>[2x]MAHHHHHHVDDDDKMVHHDGFQTVKATIDWEHPMFKLYEKAKRNGKWNPADIDFSQDQKDFASLTSEEKISALPLVAGFSAGEEAATLDILPMAHALARQGRLEDVLFLTTFMHDEAKHVEMFSRWQQAVGIGQMDLSVFHNDHYKRIFYEALPEAMNRLYADDSPEAVIRAATVYNMIVEGTLAESGYYTFRQIYKKAGLFPGLLQGIDYLNMDEGRHIQFGIYTIQRIVNEDERYYELFIRYMDELWPHVIGYVDYLTELGKRQQQLARTYALEIDYDLLRHYVIKQFNLRKKQISRTKRVDVVEGLEKTAAES

The heterodinuclear Mn/Fe cofactor is found in the R2 subunits of subclass Ic ribonucleotide reductases (denoted as R2c) as well as a related group of proteins known as R2-like ligand-binding oxidases (R2lox). Although the physiological function of R2lox proteins is not known, the cofactor catalyzes formation of a tyrosine–valine ether cross-link in the protein scaffold. Two proteins from this group have been characterized to date, homologs from Mycobacterium tuberculosis and Geobacillus kaustophilus. Both contain the ether cross-link, and both co-purify from heterologous expression hosts with a long-chain fatty acid ligand bound in a hydrophobic channel leading from the protein surface to the active site, hence the name ligand-binding oxidase. The two metal ions are bound next to each other in octahedral geometry by two histidines and four glutamates, with the manganese ion occupying the N-terminal metal-binding site 1.

The cross-linking valine, which is completely conserved across the R2lox group, was changed to an alanine, isoleucine or leucine (V72A/I/L). Crystal structures were obtained of all three R2lox point mutants in the non-activated reduced and the oxidized resting state by soaking apo-protein crystals with MnII and FeII under anoxic or aerobic conditions, respectively. The V72A/L mutations were found to have little effect on the global structures of the reduced and oxidized resting states, but an ether cross-link was not formed in the oxidized state. The mutations affect the position of the fatty acid ligand in comparison to the wild-type, likely due to decreased or increased steric constraints in the respective active site. Since the outward shift of E202 in the oxidized state reduces the steric strain on the active site, the effect is much more pronounced in the reduced state structures, but is also observed in the oxidized state. In reduced V72A-R2lox, however, the fatty acid ligand is less disordered than in the wild-type and clearly bridges the metal ions as a monodentate rather than a bidentate ligand, with the second carboxyl oxygen pointing towards A72, whereas in V72L-R2lox, the fatty acid ligand is displaced upwards in the channel in the reduced state and does not coordinate the metal ions at all. Primary or secondary carbon atoms, however, cannot be oxidized by the Mn/Fe cofactor of R2lox, likely because the resulting alkyl radical would be too unstable.> WRKKRKDAKNNEVSFSQIKPKKSKLIRVENFEAYFKKQQADSNCGFAEEYEDLKLIGISLPKYAAEIAENRGKNRYNNVLPYDISRVKLS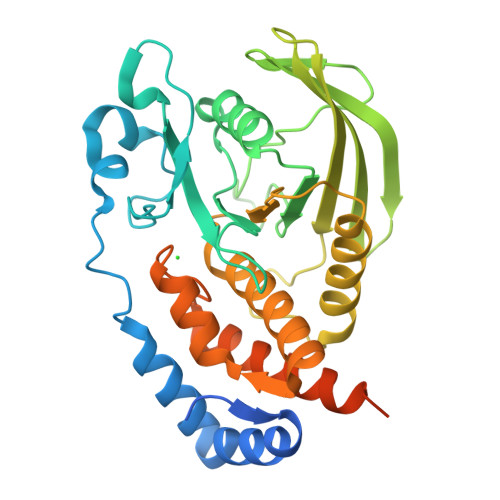VQTHSTDDYINANYMPGYHSKKDFIATQGPLPNTLKDFWRMVWEKNVYAIVMLTKCVEQGRTKCEEYWPSKQAQDYGDITVAMTSEVVLPEWTIRDFVVKNMQSSESHPLRQFHFTSWPDHGVPDTTDLLINFRYLVRDYMKQIPPESPILVHCSAGVGRTGTFIAIDRLIYQIENENTVDVYGIVYDLRMHRPLMVQTEDQYVFLNQCVLDIIRAQKDSKVDLIYQNTTAMTIYENLERVSMFGKANGYIA> SGKLRLYKEKLEGYNRFYSIVKTIKMVTLAKYRAAQGRIRTR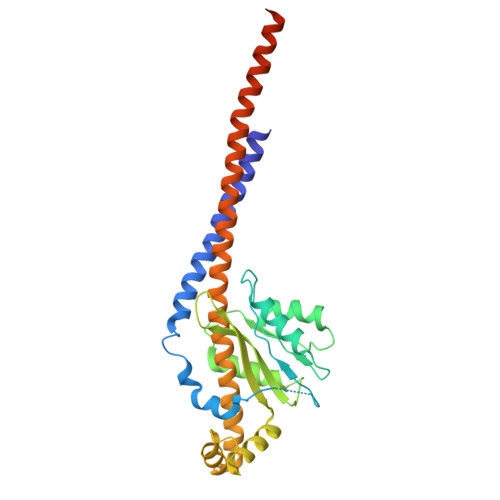DFSLRYTELAFSKPQASRDAVAAAKNALVYIPITTNRGSCGALNSNIVRCIDSVVSSKMVLMPVGKRGIDSFSKLYPDEFRYGIINDMKESMHFGYATFVIENAYEVSKDADRYQVIFNRFVSAGVQRNAVYNIPSYEKWKEDLADAASSDNQKNRYLFANALQNEEEQLIRDFFDFHAALAVLNAVGENELSEQAARLVAVEGQLTNISSLQQRTSSLYNKTRQFGITAALIEILSAMSSLEGNAMKGVRRNKFWEGAVTK> MASSRCPAPRGCRCLPGASLAWLGTVLLLLADWVLLRTALPRIFSLLVPTALPLLRVWAVGLSRWAVLWLGACGVLRATVGSKSENAGAQGWLAALKPLAAALGLALPGLALFRELISWGAPGSADSTRLLHWGSHPTAFVVSYAAALPAAALWHKLGSLWVPGGQGGSGNPVRRLLGCLGSETRRLSLFLVLVVLSSLGEMAIPFFTGRLTDWILQDGSADTFTRNLTLMSILTIASAVLEFVGDGIYNNTMGHVHSHLQGEVFGAVLRQETEFFQQNQTGNIMSRVTEDTSTLSDSLSENLSLFLWYLVRGLCLLGIMLWGSVSLTMVTLITLPLLFLLPKKVGKWYQLLEVQVRESLAKSSQVAIEALSAMPTVRSFANEEGEAQKFREKLQEIKTLNQKEAVAYAVNSWTTSISGMLLKVGILYIGGQLVTSGAVSSGNLVTFVLYQMQFTQAVEVLLSIYPRVQKAVGSSEKIFEYLDRTPRCPPSGLLTPLHLEGLVQFQDVSFAYPNRPDVLVLQGLTFTLRPGEVTALVGPNGSGKSTVAALLQNLYQPTGGQLLLDGKPLPQYEHRYLHRQVAAVGQEPQVFGRSLQENIAYGLTQKPTMEEITAAAVKSGAHSFISGLPQGYDTEVDEAGSQLSGGQRQAVALARALIRKPCVLILDDATSALDANSQLQVEQLLYESPERYSRSVLLITQHLSLVEQADHILFLEGGAIREGGTHQQLMEKKGCYWAMVQAPADAPE;> MRLPDLRPWTSLLLVDAALLWLLQGPLGTLLPQGLPGLWLEGTLRLGGLWGLLKLRGLLGFVGTLLLPLCLATPLTVSLRALVAGASRAPPARVASAPWSWLLVGYGAAGLSWSLWAVLSPPGAQEKEQDQVNNKVLMWRLLKLSRPDLPLLVAAFFFLVLAVLGETLIPHYSGRVIDILGGDFDPHAFASAIFFMCLFSFGSSLSAGCRGGCFTYTMSRINLRIREQLFSSLLRQDLGFFQETKTGELNSRLSSDTTLMSNWLPLNANVLLRSLVKVVGLYGFMLSISPRLTLLSLLHMPFTIAAEKVYNTRHQEVLREIQDAVARAGQVVREAVGGLQTVRSFGAEEHEVCRYKEALEQCRQLYWRRDLERALYLLVRRVLHLGVQMLMLSCGLQQMQDGELTQGSLLSFMIYQESVGSYVQTLVYIYGDMLSNVGAAEKVFSYMDRQPNLPSPGTLAPTTLQGVVKFQDVSFAYPNRPDRPVLKGLTFTLRPGEVTALVGPNGSGKSTVAALLQNLYQPTGGQVLLDEKPISQYEHCYLHSQVVSVGQEPVLFSGSVRNNIAYGLQSCEDDKVMAAAQAAHADDFIQEMEHGIYTDVGEKGSQLAAGQKQRLAIARALVRDPRVLILDEATSALDVQCEQALQDWNSRGDRTVLVIAHRLQTVQRAHQILVLQEGKLQKLAQL;> RRYQSTEL

Peptides destined for display are first delivered into the endoplasmic reticulum (ER) by the transporter associated with antigen processing (TAP). TAP is a heteromeric ATP-binding cassette (ABC) transporter comprising two subunits, TAP1 and TAP2. Each subunit has an N-terminal transmembrane domain (TMD0) that interacts with other components of the larger peptide-loading complex, a six-transmembrane helical domain (TMD) that forms the translocation pathway, and a nucleotide-binding domain (NBD) that hydrolyzes ATP. In this study, we analyzed the structure of TAP in the presence and absence of peptides. These structures show that TAP suspends peptides across its transmembrane cavity, anchoring their termini in two distal binding pockets primarily through their backbone atoms.

We created an 8-mer modified b27 peptide (b27′) lacking the central lysine at position five, and two 7-mer modified b27 peptides, each lacking the lysine as well as the adjacent glutamine (b27″) or serine [b27″(Q)]. The 8-mer B27′ increased the ATPase activity of TAP to a slightly greater extend compared to b27. Structural analysis revealed that the N and C termini of b27′ bind to TAP using the same interactions as b27. Because the peptide is shorter than b27 by 2 Å, it induces a minor contraction of the translocation pathway. Intriguingly, the arrangement of the TM helices is more similar to the a2- and c4-bound structures than the b27-bound structure. Consequently, the lateral opening seen in the b27-bound structure is no longer present, and the ER luminal gate is entirely closed. NBD separation is greatest in the apo structure (53 Å), and reduced in the presence of peptides to between 35 Å (for the 14-mer peptide) and 27 Å (for the 8-mer peptide). The shortest distance we observed between the N- and C-binding pockets was 25 Å in the 8-mer peptide-bound structure. This suggests that a minimum of eight residues is required for a fully extended peptide to be effectively engaged by both binding pockets and initiate high-affinity binding and subsequent transport into the ER lumen.methyl 7-{[2-({N-[(2S)-2-hydroxy-3,3-dimethyl-4-(phosphonooxy)butanoyl]-beta-alanyl}amino)ethyl]sulfanyl}-7-oxoheptanoate 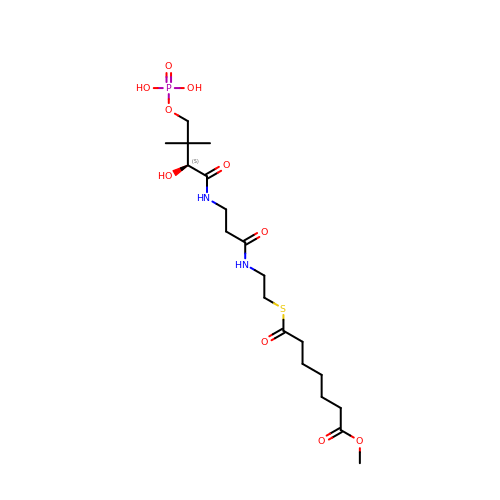| C19 H35 N2 O10 P S | HCFLUHFHCAMJNF-QGZVFWFLSA-N> SPPKRLTREAMRNYLKERGDQTVLILHAKVAQKSYGNEKRFFCPPPCVYLMGSGWKKKKEQMERDGCSEQESQPCAFIGIGNSDQEMQQLNLEGKNYCTAKTLYISDSDKRKHFMLSVKMFYGNSDDIGVFLSKRIKVISKPSKKKQSLKNADLCIASGTKVALFNRLRSQTVSTRYLHVEGGNFHASSQQWGAFYIHLLDDDESEGEEFTVRDGYIHYGQTVKLVCSVTGMALPRLIIRKVDKQTALLDADDPVSQLHKCAFYLKDTERM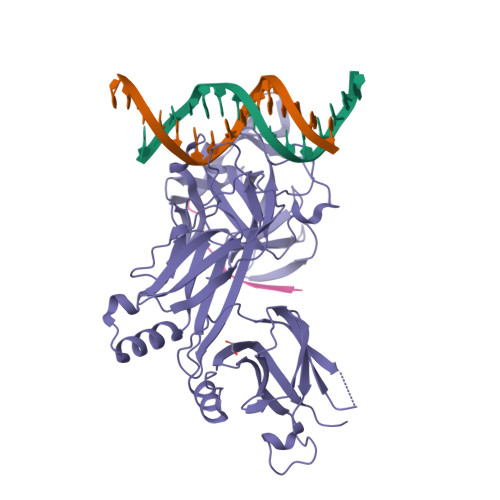YLCLSQERIIQFQATPCPKEQNKEMINDGASWTIISTDKAEYTFYEGMGPVLAPVTPVPVVESLQLNGGGDVAMLELTGQNFTPNLRVWFGDVEAETMYRCGESMLCVVPDISAFREGWRWVRQPVQVPVTLVRNDGVIYSTSLTFTYTPEP;> KKATATTWMVPTA> CVEEVTTTLEETKFLTENLLLYIDINGNLHPDSATLVSDIDITFLKKDAPYIVGDVVQEGVLTAVVIPTKKAGGTTEMLAKALRKVPTDNYITTYPGQGCNGYTVEEAKTVLKKCKSAFYILPSIISNEKQEILGTVSWNLREMLAHAEETRKLMPVCVETKAIVSTIQRKYKGIKIQEGVVDYGARFYFYTSKTTVASLINTLNDLNETLVTMPLGYVTHGLNLEEAARCMRSLKVPATVSVSSPDAVTAYNGYLTSSS

Among all SARS-CoV-2 encoded proteins, the nonstructural protein 3 (nsp3) is the largest, and it participates in many essential steps in the virus life cycle. In addition to the CoV-conserved domains of nsp3, SARS-CoV-2 nsp3 harbors a “SARS-Unique Domain” (SUD), which was first identified in the SARS-CoV genome. SUD contains three subdomains; there are two macrodomains, Mac2 and Mac3, that are followed by a frataxin-like Domain Preceding Ubl2 and PL2pro (DPUP). SUD-core does not possess enzymatic activity; rather, it functions as a binding module for viral and host molecules.

We expressed a nsp3 fragment (residue 413–676) comprising SUD-N and SUD-M domains, denoted SARS-CoV-2 SUD-core. Although this fragment was highly soluble, it failed to crystalize despite considerable efforts. We reasoned that the lack of disulfide bond between SUD-N and SUD-M might confer high flexibility and prevented the crystallization. Therefore, we engineered a disulfide bond in SARS-CoV-2 SUD-core based on SARS-CoV SUD-core; the resulting mutant containing double mutations L516C-Y647C was denoted SARS-CoV-2 SUD-core-CC. To crystalize SARS-CoV-2 SUD-core-CC, we avoided using reducing reagents in latter stages of purification to promote disulfide bond formation. The protein was finally exchanged into an oxidative buffer and incubated overnight before crystallization screening. Initial SUD crystals diffracted to ~ 2.3 Å, and the crystals were gradually improved by optimizing crystallization conditions. SUD-core-CC comprises tandem SUD-N and SUD-M macrodomains connected by a flexible loop region. Both SUD-N and SUD-M adopt the typical ‘macro fold’, a mixed six-stranded β-plane is sandwiched by short α-helices and connecting loops on both sides. We clearly observed the engineered disulfide bond between L561C and Y647C, tethering SUD-N and SUD-M together. (2) We did not observe the SARS-CoV SUD-like dimers in the crystal structure of SARS-CoV-2 SUD-core-CC, and PISA software did not identify any other quaternary structures larger than monomers, consistent with the results of size-exclusion chromatography and analytical ultracentrifugation, demonstrating that the SARS-CoV-2 SUD-core formed monodispersed monomers in solution.>STTQYDHKESCNGLYYQGSCYILHSDYQMFSDAAANCTAESSTLPNKSDVMITWLIDYVEDTWGSDGNPITKTTSDYQDSDVSQEVRK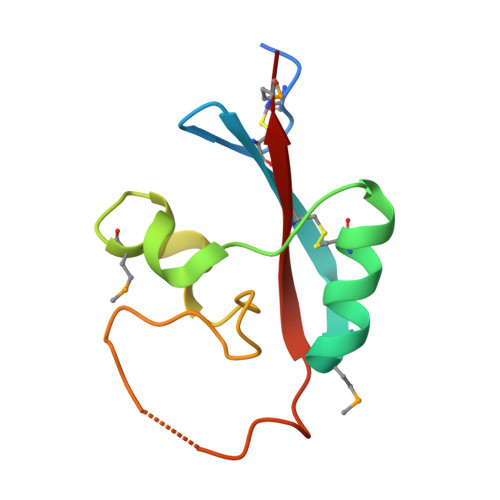YFCVKTMN[2x]>[2x]LDG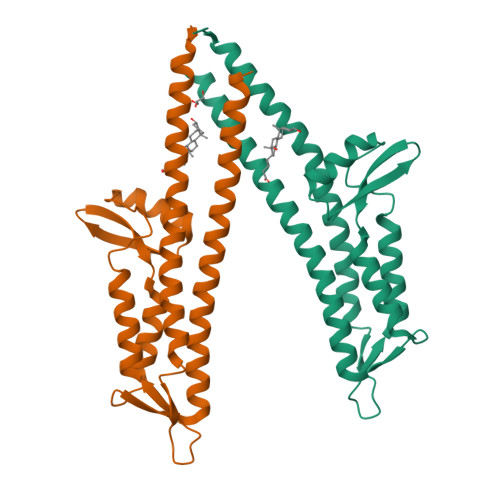DQMISHRELWAKIANSINDINEYLKVYEHAVSSYTQMYQDFSAVLSSLAGWISPGGNDGNSVKLQVNSLKKALEELKEKYKDKPLYPANNTVSQEQANKWLTELGGTIGKVSQKNGGYVVSINMTPIDNMLKSLDNLGGNGEVVLDNAKYQAWNAGFSAEDETMKNNLQTLVQKYSNANSIFDNLVKVLSSTISS> TVIEKRIVIDGDGDIDHDQALAQAIREAREQHPDMSVTRVVVNKETELAEEGED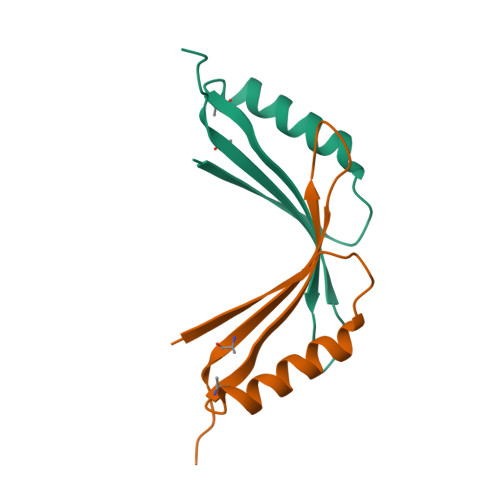RTRQIINITMTKKLDVW;> VIEKRIVIDGDGDIDHDQALAQAIREAREQHPDMSVTRVVVNKETELAEEGEDRTRQIINITMTKKLDVW Tumor-suppressor let-7 pre-microRNAs (miRNAs) are regulated by terminal uridylyltransferases TUT7 and TUT4 that either promote let-7 maturation by adding a single uridine nucleotide to the pre-miRNA 3′ end or mark them for degradation by the addition of multiple uridines. Oligo-uridylation is increased in cells by enhanced TUT7/4 expression and especially by the RNA-binding pluripotency factor LIN28A. TUT4 and TUT7 are multidomain enzymes whose specific targeting of RNAs makes use of three zinc fingers, combined with two copies of a nucleotidyltransferase domain (NTD), one inactive in the N-terminal half of the polypeptide (pseudo-NTD) and one active in the C-terminal half. Our structures reveal that pre-miRNAs engage the enzymes in fundamentally different ways depending on the presence of LIN28A, which clamps them onto the TUTs to enable processive 3′ oligo-uridylation.

In conformation I, most of the pre-let-7g could be resolved. In this conformation, the RNA stem interacts with the TUT7 LIM, while the let-7g 49AGGAG53 region coordinates with the zinc finger of TUT7 and ZK domain of LIN28A, forming a stable ternary complex35. Furthermore, despite clear density representing the pre-element (the apical loop and short stem region preceding later removed by Dicer action), no density was observed for the CSD of LIN28A, presumably due to the relative flexibility between the LIM + LIN28A and pre-let-7g. Based on the position of the RNA, this complex is believed to represent the initial step in oligo-uridylation, a ‘capture’ state in which the pre-let-7 has begun association with TUT7 but not yet completed its engagement. By contrast, comparison of TUT7 ternary conformations I and II finds no change in the relative positions of the palm and fingers subdomains of the LIM while the zinc finger binding the pre-let-7 stem moves substantially about a 16.8° rotation of the linking helix. The binding mode and overall conformation of the pre-let-7g miRNA appears to be remarkably consistent in all three LIN28A-containing complexes, apparently due to the LIM/LIN28A clasp and other key interfaces shown by mutational data to be the specific interactions responsible for ensuring efficient and processive oligo-uridylation.

> MGDTAKPYFVKRTKDRGTMDDDDFRRGHPQQDYLIIDDHAKGHGSKMEKGLQKKKITPGNYGNTPRKGPCAVSSNPYAFKNPIYSQPAWMNDSHKDQSKRWLSDEHTGNSDNWREFKPGPRIPVINRQRKDSFQENEDGYRWQDTRGCRTVRRLFHKDLTSLETTSEMEAGSPENKKQRSRPRKPRKTRNEENEQDGDLEGPVIDESVLSTKELLGLQQAEERLKRDCIDRLKRRPRNYPTAKYTCRLCDVLIESIAFAHKHIKEKRHKKNIKEKQEEELLTTLPPPTPSQINAVGIAIDKVVQEFGLHNENLEQRLEIKRIMENVFQHKLPDCSLRLYGSSCSRLGFKNSDVNIDIQFPAIMSQPDVLLLVQECLKNSDSFIDVDADFHARVPVVVCREKQSGLLCKVSAGNENACLTTKHLTALGKLEPKLVPLVIAFRYWAKLCSIDRPEEGGLPPYVFALMAIFFLQQRKEPLLPVYLGSWIEGFSLSKLGNFNLQDIEKDVVIWEHTDSAAGDTGITKEEAPRETPIKRGQVSLILDVKHQPSVPVGQLWVELLRFYALEFNLADLVISIRVKELVSRELKDWPKKRIAIEDPYSVKRNVARTLNSQPVFEYILHCLRTTYKYFALPHKITKSSLLKPLNAITCISEHSKEVINHHPDVQTKDDKLKNSVLAQGPGATSSAANTCKVQPLTLKETAESFGSPPKEEMGNEHISVHPENSDCIQADVNSDDYKGDKVYHPETGRKNEKEKVGRKGKHLLTVDQKRGEHVVCGSTRNNESESTLDLEGFQNPTAKECEGLATLDNKADLDGESTEGTEELEDSLNHFTHSVQGQTSEMIPSDEEEEDDEEEEEEEEPRLTINQREDEDGMANEDELDNTYTGSGDEDALSEEDDELGEAAKYEDVKECGKHVERALLVELNKISLKEENVCEEKNSPVDQSDFFYEFSKLIFTKGKSPTVVCSLCKREGHLKKDCPEDFKRIQLEPLPPLTPKFLNILDQVCIQCYKDFSPTIIEDQAREHIRQNLESFIRQDFPGTKLSLFGSSKNGFGFKQSDLDVCMTINGLETAEGLDCVRTIEELARVLRKHSGLRNILPITTAKVPIVKFFHLRSGLEVDISLYNTLALHNTRLLSAYSAIDPRVKYLCYTMKVFTKMCDIGDASRGSLSSYAYTLMVLYFLQQRNPPVIPVLQEIYKGEKKPEIFVDGWNIYFFDQIDELPTYWSECGKNTESVGQLWLGLLRFYTEEFDFKEHVISIRRKSLLTTFKKQWTSKYIVIEDPFDLNHNLGAGLSRKMTNFIMKAFINGRRVFGIPVKGFPKDYPSKMEYFFDPDVLTEGELAPNDRCCRICGKIGHFMKDCPMRRKVRRRRDQEDALNQRYPENKEKRSKEDKEIHNKYTEREVSTKEDKPIQCTPQKAKPMRAAADLGREKILRPPVEKWKRQDDKDLREKRCFICGREGHIKKECPQFKGSSGSLSSKYMTQGKASAKRTQQES;> MGSVSNQQFAGGCAKAAEEAPEEAPEDAARAADEPQLLHGAGICKWFNVRMGFGFLSMTARAGVALDPPVDVFVHQSKLHMEGFRSLKEGEAVEFTFKKSAKGLESIRVTGPGGVFCIGSERRPKGKSMQKRRSKGDRCYNCGGLDHHAKECKLPPQPKKCHFCQSISHMVASCPLKAQQGPSAQGKPTYFREEEEEIHSPTLLPEAQN>LSPAELHADSIVIDGLIIAKWNRELFEDMRKGGLTAANCTVSVWEGFQATVNNITASNKLIRDNSDLVIPVRSTADIRKAKEQGKTGILYGFQNAHAFEDQIGYVEVFKQLGVGIVQMCYNTQNLVGTGCYERDGGLSGFGREIVAEMNRVGIMCDLSHVGSKTSEEVILESKKPVCYSHCLPSGLKEHPRNKSDEELKFIADHGGFVGVTMFAPFLKKGIDSTIDDYAEAIEYVMNIVGEDAIGIGTDFTQGHGH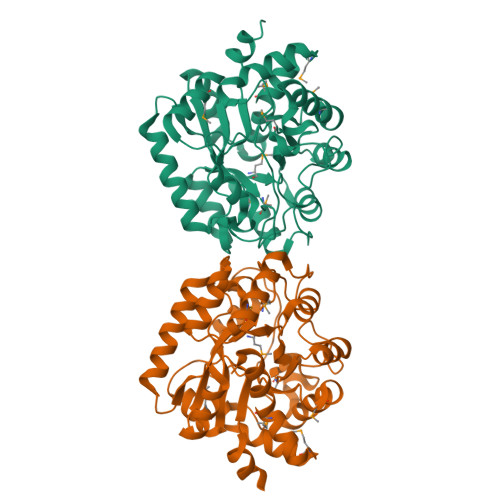DFFEWLTHDKGYARRLTNFGKIVNPLGIRTVGEFPNLTETLLKRGMPERVVRKVMGENWVRVLRDVWGE[2x]>SMGKLSEQLKHCNGILKELLSKKHAAYAWPFYKPVDASALGVHDYHDIIKHPMDLSTVKRKMENRDYRDAQEFAA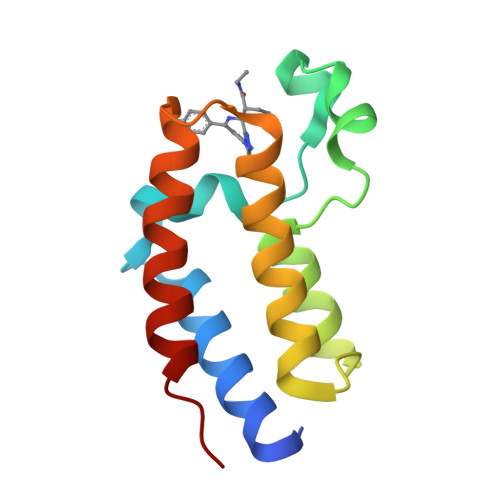DVRLMFSNCYKYNPPDHDVVAMARKLQDVFEFRYAKMPD[2x]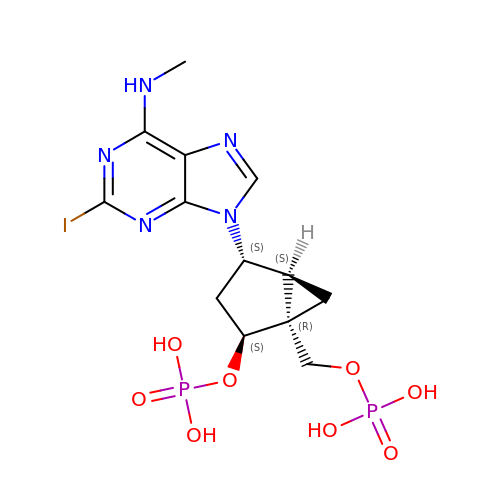[(1R,2S,4S,5S)-4-[2-iodo-6-(methylamino)-9H-purin-9-yl]-2-(phosphonooxy)bicyclo[3.1.0]hex-1-yl]methyl dihydrogen phosphate | C13 H18 I N5 O8 P2 | NMVWLEUONAKGCD-SMWKGLLFSA-N Intimin is a 94 kDa outer membrane protein, essential for the intimate attachment of bacterial cells to the host cell surface, followed by actin pedestal formation. Intimin is classified as an inverse autotransporter, a subclass of the type 5 secretion system that transports the C-terminal extracellular region or passenger through the lumen of the N-terminal β-barrel located in the outer membrane. The intimin passenger forms a rod-like extension consisting of four tandem bacterial immunoglobulin-like (Big) domains (subdomains D00–D0–D1–D2) capped by a C-terminal C-type lectin-like domain (D3). Here, we describe the crystal structures of the combined intimin domains D00–D0 and D0–D1 from the EPEC strain E2348/69 determined at 1.5 Å and 1.8 Å resolution, respectively.

The structure of D00–D0 has an elongated conformation, spanning 78 Å between the N- and C-termini. The subdomain D00 also exhibits an IgSF fold with a β-sandwich, yet it shows distinct structural differences when compared to the s-type fold seen in subdomains D0 and D1. In addition to the two common β-sheets, β-strands A1 and B2 form a separate small β-sheet due to shortened β-strands D and E. The presence of a third β-sheet in an Ig-fold is not novel as it has been previously described in Ig-domain subtype C425. The β-sandwich of D00 is additionally disrupted in strand C by a short α-helix induced by residue Pro515. A structural similarity search with the D00 structure on PDBeFold revealed similarity to the outermost extracellular domains of several Cadherin types (EC). The D00–D0 connector adopts an S-shaped conformation connecting the D0 and the D00 domains through a hydrogen bond network and solvent-free dry interface. The tight interaction between these two key residues leads to the formation of a classical type I turn in the connector. The asymmetric unit of D00–D0 crystals contained six molecules. The sidechain rotamer of all the implicated residues and thus the hydrogen bond network of the D00–D0 connector region is conserved in all six molecules. OLIGOMER results had a better fit to experimental data (χ2 = 2.45 for merged file) and revealed that the majority of D00–D0 is present in the elongated conformation as shown in the crystal structure.

>[6x]SKQDILSLNIPHDINGTERSTQKIQLIVKSKYGLDRIVWDDSALRSQGGQIQHSGSQSAQDYQAILPAYVQGGSNVYKVTARAYDRNGNSSNNVLLTITVLSNGQVVDQVGVTDFTADKTSAKADGTEAITYTATVKKNGVAQANVPVSFNIVSGTAVLSANSANTNGSGKATVTLKSDKPGQVVVSAKTAEMTSALNANAVIFVDQ>HMASMTGGQQMGRGSDFGDIEERGKILVSLMYSTQQGGLIVGIIRCVHLAAMDAN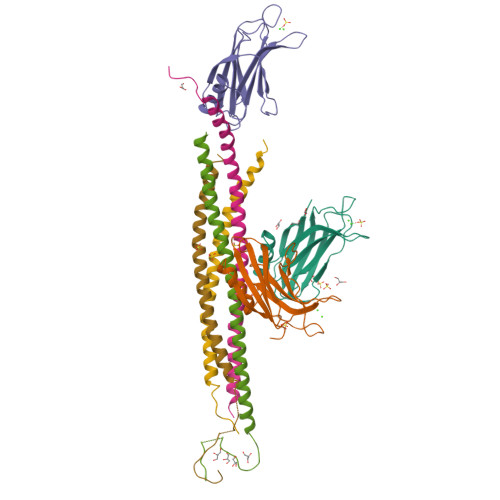GYSDPFVKLWLKPDMGKKAKHKTQIKKKTLNPEFNEEFFYDIKHSDLAKKSLDISVWDYDIGKSNDYIGGCQLGISAKGERLKHWYECLKNKDKKIERWHQLQNENH[3x];>[2x]XXXXXGSHMASMTGGQQMGRGSEFMRNELEEMQRRADQLADESLESTRRMLQLVEESKDAGIRTLVMLDEQGEQLDRVEEGMNHINQDMKEAEKNLKDLG;>XXXXXXXXXXXXXXGSHMASMTGGQQMGRGSEFARENEMDENLEQVSGIIGNLRHMALDMGNEIDTQNRQIDRIMEKADSNKTRIDEANQRATKML[2x]>[2x]VIEKVQHIQLLQKNVRAQLVDMKRLEVDIDIKIRSCRGSCSRALAREVDLKDYEDQQKQLEQVIAK;>HQLYIDETVNSNIPTNLRVLRSILENLRSKIQKLESDVSAQMEYCRTPCTVSCNIPVVSGKECEEIIRKGGETSEMYLIQPDSSVKPYRVYCDMNTENGGWTVIQNRQDGSVDFGRKWDPYKQGFGNVATNTDGKNYCGLPGEYWLGNDKISQLTRMGPTELLIEMEDWKGDKVKAHYGGFTVQNEANKYQISVNKYRGTAGNALMDGASQLMGENRTMTIHNGMFFSTYDRDNDGWLTSDPR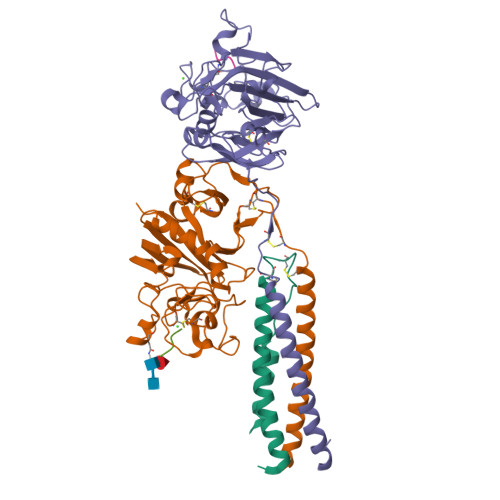KQCSKEDGGGWWYNRCHAANPNGRYYWGGQYTWDMAKHGTDDGVVWMNWKGSWYSMRKMSMKIRPFFPQQ[2x];>[2x]YEASILTHDSSIRYLQEIYNSNNQKIVNLKEKVAQLEAQCQEPCKDTVQIHDITGKDCQDIANKGAKQSGLYFIKPLKANQQFLVYCEIDGSGNGWTVFQKRLDGSVDFKKNWIQYKEGFGHLSPTGTTEFWLGNEKIHLISTQSAIPYALRVELEDWNGRTSTADYAMFKVGPEADKYRLTYAYFAGGDAGDAFDGFDFGDAPSAKFFTSHNGMQFSTWDNDNDKFEGNCAEQDGSGWWMNKCHAGHLNGVYYQGGTYSKASTPNGYDNGIIWATWKTRWYSMKKTTMKIIPFNRLTIGEGQQHHLGGAK;>GPRP[4x]> MDLPYYHGRLTKQDCETLLLKEGVDGNFLLRDSESIPGVLC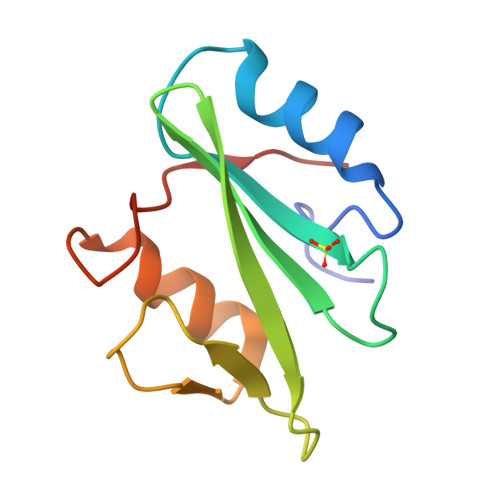LCVSFKNIVYTYRIFREKHGYYRIQTAEGSPKQVFPSLKELISKFEKPNQGMVVHLLKPIKRT>[2x]GGSIDETRAHLLLKEKMMRLGGRLVLNTKEELANERLMTLKIAEMKEAMRTLIFPPSMHFFQAKHLIERSQVFNILRMMPKGAALHLHDIGIVTMDWLVRNVTYRPHCHICFTPRGIMQFRFAHPTPRPSEKCSKWILLEDYRKRVQNVTEFDDSLLRNFTLVTQHPEVIYTNQNVVWSKFETIFFTISGLIHYAPVFRDYVFRSMQEFYEDNVLYMEIRARLLPVYELSGEHHDEEWSVKTYQEVAQKFVETHPEFIGIKIIYSDHRSKDVAVIAESIRMAMGLRIKFPTVVAGFDLVGHEDTGHSLHDYKEALMIPAKDGVKLPYFFHAGETDWQGTSIDRNILDALMLNTTRIGHGFALSKHPAVRTYSWKKDIPIEVCPISNQVLKLVSDLRNHPVATLMATGHPMVISSDDPAMFGAKGLSYDFYEVFMGIGGMKADLRTLKQLAMNSIKYSTLLESEKNTF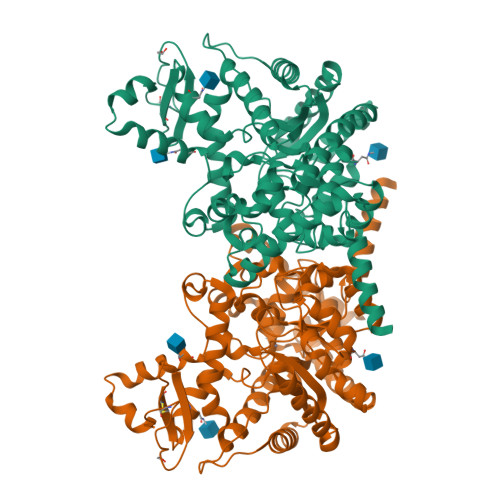MEIWKKRWDKFIADVATKGSLHHILDAQKMVWNHRHHHHHH>[2x]MSLRITRLTVFHLDLPLAKPYWLSGGRLKFDRLDSTYLRIDTDEG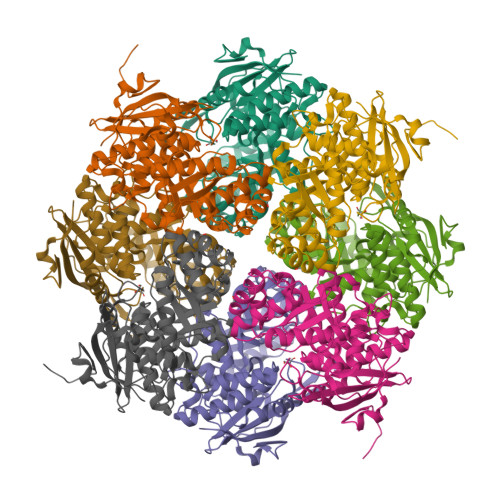VTGWGEGCPWGHSYLPAHGPGLRAGIATLAPHLLGLDPRSLDHVNRVMDLQLPGHSYVKSPIDMACWDILGQVAGLPLWQLLGGEAATPVPINSSISTGTPDQMLGLIAEAAAQGYRTHSAKIGGSDPAQDIARIEAISAGLPDGHRVTFDVNRAWTPAIAVEVLNSVRARDWIEQPCQTLDQCAHVARRVANPIMLDECLHEFSDHLAAWSRGACEGVKIKPNRVGGLTRARQIRDFGVSVGWQMHIEDVGGTALADTAALHLAASTPEANRLASWLGHAHLADDPIPGQGARNRDGLATPPSAPGLGVIPDPEALGRPVASYDEGHHHHHH>[2x]QKPGETKEVHPQLTTFRCTKRGGCKPATNFIVLDSLSHPIHRAEGLGPGGCGDWGNPPPKDVCPDVESCAKNCIMEGIPDYSQYGVTTNGTSLRLQHILPDGRVPSPRVYLLDKTKRRYEMLHLTGFEFTFDVDATKLPCGMNSALYLSEMHPTGAKSKYNPGGAYYGTGYCDAQCFV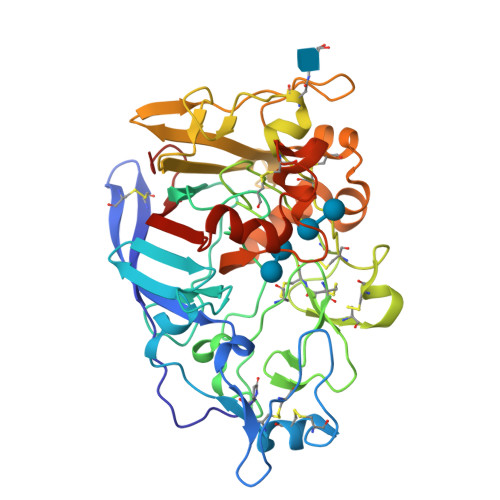TPFINGLGNIEGKGSCCNSMDIWEANSRASHVAPHTCNKKGLYLCEGEECAFEGVCDKNGCGWNNYRVNVTDYYGRGEEFKVNTLKPFTVVTQFLANRRGKLEKIHRFYVQDGKVIESFYTNKEGVPYTNMIDDEFCEATGSRKYMELGATQGMGEALTRGMVLAMSIWWDQGGNMEWLDHGEAGPCAKGEGAPSNIVQVEPFPEVTYTNLRWGEIGSTYQELQ> GSHMGSPNSPLKDS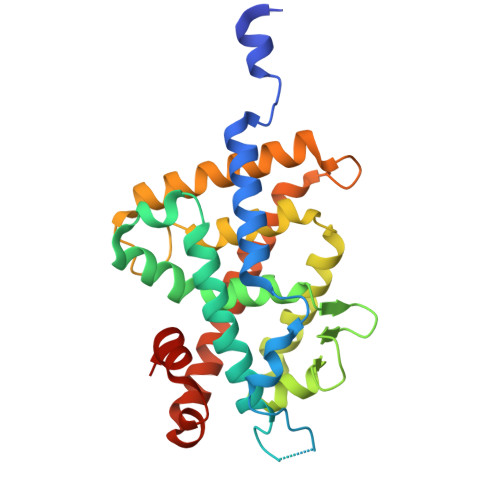LRPKLSEEQQHIIAILLDAHHKTYDPTYADFRDFRPPVRMDGSTGSVTLDLSPLSMLPHLADLVSYSIQKVIGFAKMIPGFRDLTSDDQIVLLKSSAIEVIMLLSNQSFTMDDMSWDCGSQDYKYDVTDVSKAGHTLELIEPLIKFQVGLKKLNLHEEEHVLLMAICIVSPDRPGVQDAKLVEAIQDRLSNTLQTYIRCRHPPPGSHQLYAKMIQKLADLRSLNEEHSKQYRSLSFQPENSMKLTPLVLEVFGNEIS> MASNYNSGLKIGAWVGTQPSESAIKSFQELQGRKLDIVHQFINWSTDFSWVRPYADAVYNNGSILMITWEPWEYNTVDIKNGKADAYITRMAQDMKAYGKEIWLRPLHEANGDWYPWAIGYSSRV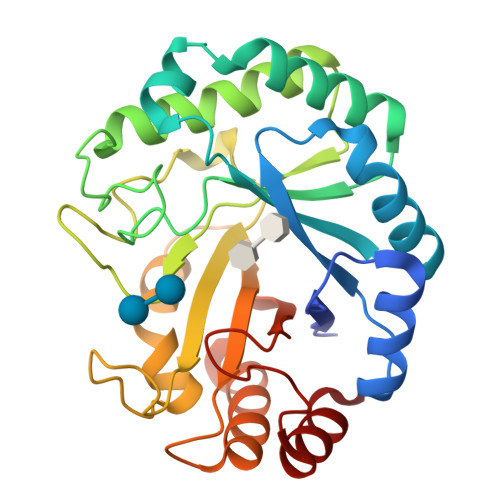NTNETYIAAFRHIVDIFRANGATNVKWVFNVNCDNVGNGTSYLGHYPGDNYVDYTSIDGYNWGTTQSWGSQWQSFDQVFSRAYQALASINKPIIIAEFASAEIGGNKARWITEAYNSIRTSYNKVIAAVWFHENKETDWRINSSPGALAAYREAIGA> SIIQVFFIAGRTDEQKERLIGALTDAAV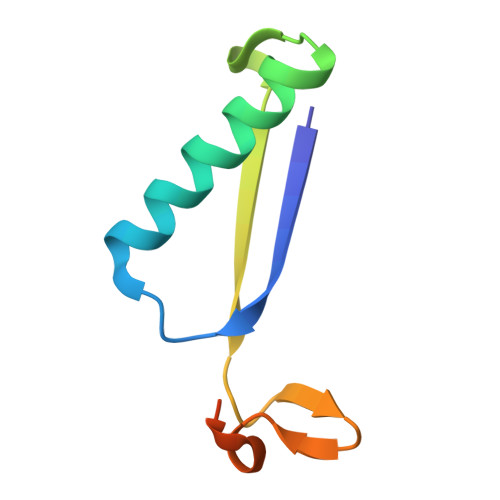KTIGIDRSDVRVILKDIPNTEYGIAGKTAKSLGRGTGRSPAGS> MRGSLPLLFNPVLPPSTARLRLLTYPMALAQPHATVPLIQPTIDGTHDGRNGATVSLRTQARMHGTADGTMATAGDSSQNNSVMDSPRWLRNPDELCVAALRRSRDVNKINSYVATYKFDDPQWAPLLLPEVTLRPQVNSTGDKPNGGNEAAADVVSVGPSVSATPESTPPPPPSSSSSSPYSCPADCVSISHNKMIMLECMSRHVNFSLRHIVQKGHGIYLIYHAQHSILQPKGLVEQSFVTCSFGIRGERLRTDIVHVGPIDAADVMELQPSEGHDHPRCCFNLYQKSDVRRGVIAVSQVEGYGT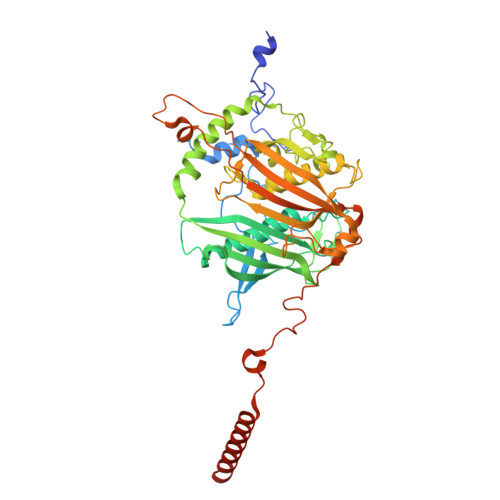WFQRKPMLWQRSRRIGALQSQLGAFAYDLVDPHEVGKWRDCEVSLLAPHMRFFRNGLNGAEAVGIIASSQVAQQRRLYLGEFEAPAITALDAVQQLAHASALRCKLVTPVVDPNGVGGTGSGSLGDENMDKHIDMETLLPLSWATRTPPPYVPLEADLPFKLQMSRPTVFAESHQQNQAYPTGGTVGSPFVRGAPMMMFEYNMHQGVDHYVYDDAPSARPMKWWSQKSNMPYSGYMYFARSGLVDRFTPSEDIPNPLEPTSKRKPLHAVVPPTKVVQERLRKYRRKQQEGHKQRRRASSGSGVSNEPDAVNRQESVSRGTCE> SKLDSYTHLSFYEKRELFRKKLREIEGPEVTLVNEVDDEPCPSLDFQFISQYRLTQGVIPPDPNFQSGCNCSSLGGCDLNNPSRCECLDDLDEPTHFAYD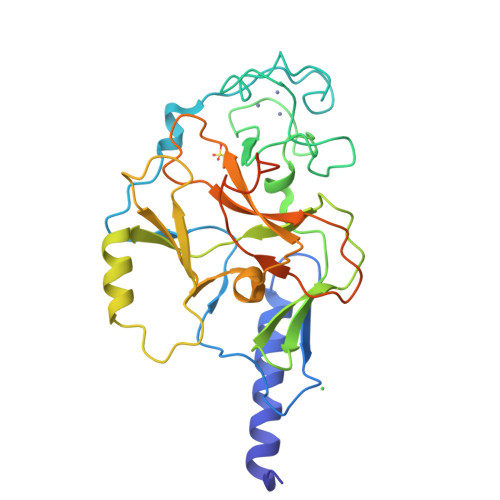AQGRVRADTGAVIYECNSFCSCSMECPNRVVQRGRTLPLEIFKTKEKGWGVRSLRFAPAGTFITCYLGEVITSAEAAKRDKNYDDDGITYLFDLDMFDDASEYTVDAQNYGDVSRFFNHSCSPNIAIYSAVRNHGFRTIYDLAFFAIKDIQPLEELTFDYAGAKDFSPVQSQKSQQNRISKLRRQCKCGSANCRGWLFG CYCLOHEXYL 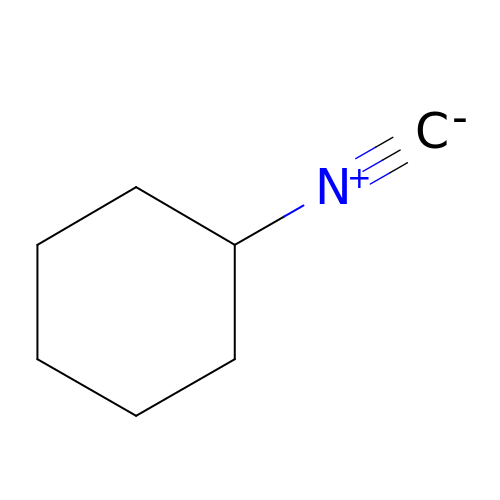ISOCYANIDE | C7 H11 N | XYZMOVWWVXBHDP-UHFFFAOYSA-N>[4x]MVRIYTLTLAPSLDSATITPQIYPEGKLRCTAPVFEPGGGGINVARAIAHLGGSATAIFPAGGATGEHLVSLLAD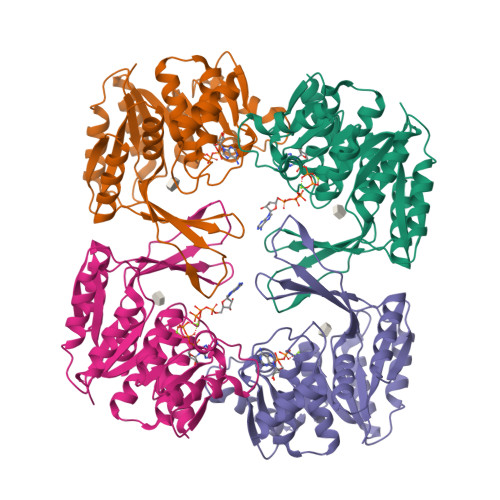ENVPVATVEAKDWTRQNLHVHVEASGEQYRFVMPGAALNEDEFRQLEEQVLEIESGAILVISGSLPPGVKLEKLTQLISAAQKQGIRCIVDSSGEALSAALAIGNIELVKPNQKELSALVNRELTQPDDVRKAAQEIVNSGKAKRVVVSLGPQGALGVDSENCIQVVPPPVKSQSTVGAGDSMVGAMTLKLAENASLEEMVRFGVAAGSAATLNQGTRLCSHDDTQKIYAYLSR>MQIYEGKLTAEGLRFGIVASRFNHALVDRLVEGAIDCIVRHGGREEDITLVRVPGSWEIPVAAGELARKEDIDAVIAIGVLIRGATPHFDYIAS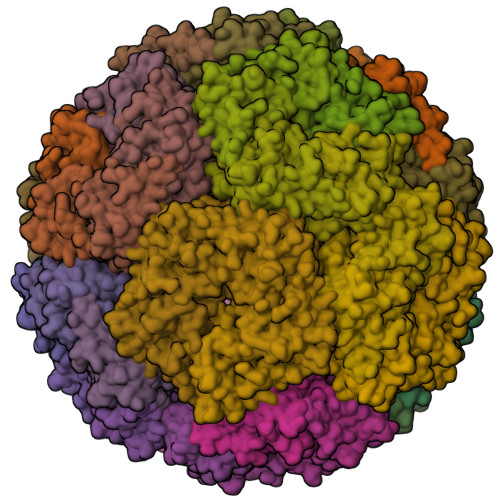EVSKGLANLSLELRKPITFGVITADTLEQAIERAGTKHGNKGWEAALSAIEMANLFKSLR[60x]>[2x]MMANRMILNETAWFGRGAVGALTDEVKRRGYQKALIVTD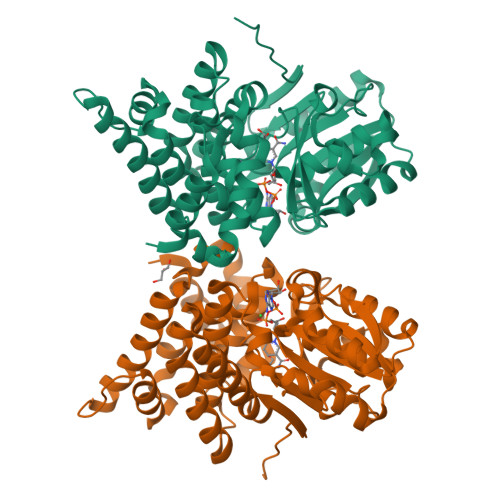KTLVQCGVVAKVTDKMDAAGLAWAIYDGVVPNPTITVVKEGLGVFQNSGADYLIAIGGGSPQDTCKAIGIISNNPEFADVRSLEGLSPTNKPSVPILAIPTTAGTAAEVTINYVITDEEKRRKFVCVDPHDIPQVAFIDADMMDGCPPALKAATGVDALTHAIEGYITRGAWALTDALHIKAIEIIAGALRGSVAGDKDAGEEMALGQYVAGMGFSNVGLGLVHGMAHPLGAFYNTPHGVANAILLPHVMRYNADFTGEKYRDIARVMGVKVEGMSLEEARNAAVEAVFALNRDVGIPPHLRDVGVRKEDIPALAQAALDDVCTGGNPREATLEDIVELYHTAWLEHHHHHH> GPRRQTIEALVPAWDSDIIFKCLCYFHTLYPGLIPLETFPPATIFNFKQKIISILEDKKAVLRGEPIKGPLPICCSKENYRRHL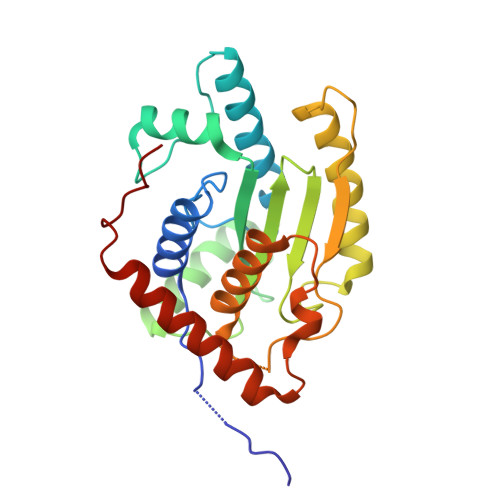QRTTLLPVFMWYHPTPKTLSDTMQTMKQLAIKGSVGASHWLLVIVDIQARRLVYFDSLYNYVMPPENMKKELQSFAQQLDQVYPAYDSKKFSVKIAAKEVIQRGSGSSCGAWCCQFLHWYLKDPLTDALNDLPVDSVERHENLASFVQACEAAVQDLPELSWPEA> MRERPHTSGHHGAGEARATAPSTVSPYGPEARAELSSRLTTLRNTLAPATNDPRYLQACGGEKLNRFRDIQCRRQTAVRADLNANYIQVGNTRTIACQYPLQSQLESHFRMLAENRTPVLAVLASSSEIANQRFGMPDYFRQSGTYGSITVESKMTQQVGLGDGIMADMYTL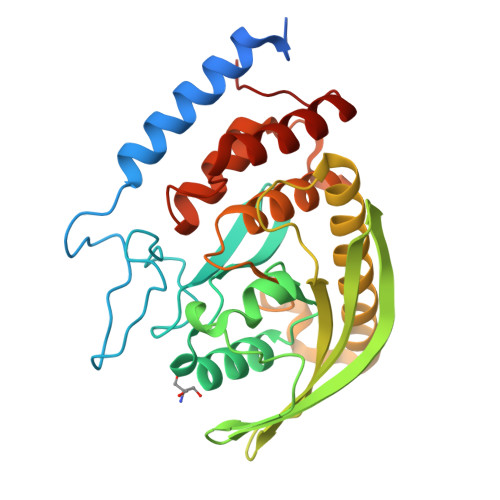TIREAGQKTISVPVVHVGNFPDQTAVSSEVTKALASLVDQTAETKRNMYESKGSSAVADDSKLRPVIHCRAGVGRTAQLIGAMCMNDSRNSQLSVEDMVSQMRVQRNGIMVQKDEQLDVLIKLAEGQGRPLLNS>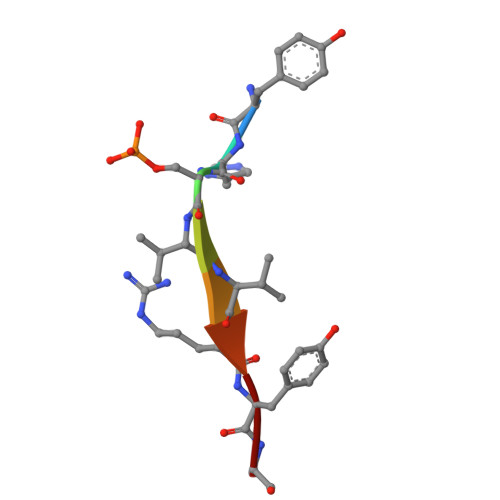 YHSVVRYA> MSTQYETQGYTINNAGRRLVVDPITRIEGHMRCEVNINDQNVITNAVSCGTMFRGLEIILQGRDPRDAWAFVERICGVCTGVHALASVYAIEDAIGIKVPDNANIIRNIMLATLWCHDHLVHFYQLAGMDWIDVLDALKADPRKTSELAQSLSSWPKSSPGYFFDVQNRLKKFVEGGQLGIFRNGYWGHPQYKLPPEANLMGFAHYLEALDFQREIVKIHAVFGGKNPHPNWIVGGMPCAINIDESGAVGAVNMERLNLVQSIITRTADFINNVMIPDALAIGQFNKPWSEIGTGLSDKCVLSYGAFPDIANDFGEKSLLMPGGAVINGDFNNVLPVDLVDPQQVQEFVDHAWYRYPNDQVGRHPFDGITDPWYNPGDVKGSDTNIQQ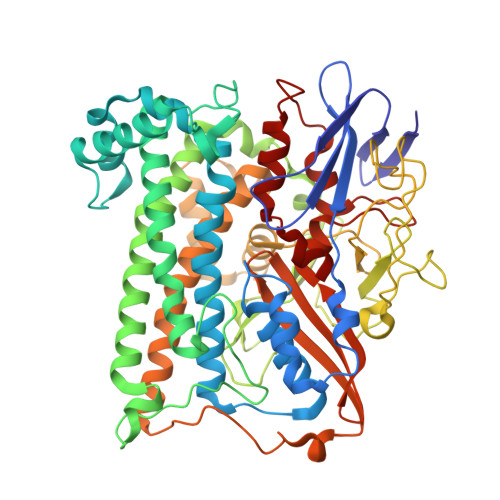LNEQERYSWIKAPRWRGNAMEVGPLARTLIAYHKGDAATVESVDRMMSALNLPLSGIQSTLGRILCRAHEAQWAAGKLQYFFDKLMTNLKNGNLATASTEKWEPATWPTECRGVGFTEAPRGALGHWAAIRDGKIDLYQCVVPTTWNASPRDPKGQIGAYEAALMNTKMAIPEQPLEILRTLHSFDPCLACSTH>[10x]MEGVDLLGFLIITLNCNVTMVGKLWFVLTMLLRMLVIVLAGRPVYQDEQERFVCNTLQPGCANVCYDVFSPVSHLRFWLIQGVCVLLPSAVFSVYVLHRGATL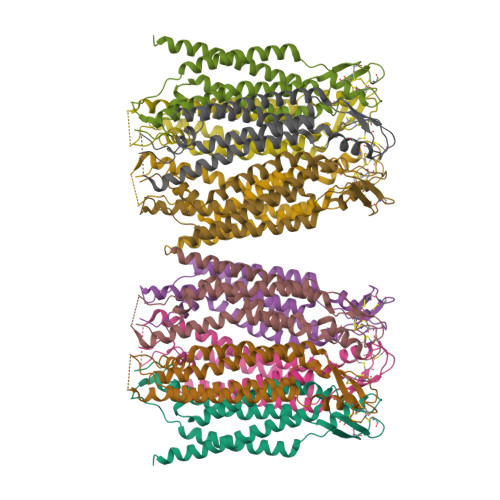AALGPRRCPDPREPASGQRRCPRPFGERGGLQVPDFSAGYIIHLLLRTLLEAAFGALHYFLFGFLAPKKFPCTRPPCTGVVDCYVSRPTEKSLLMLFLWAVSALSFLLGLADLVCSLRRRMRRRPGPPTS> MTSSVLAALLSVSIMLVQLRAEANIGTGDNVLHRAALCGIIELAGKRAKLETALPNFQNELNSILELNMTAAEPTWLDQFRDKDDRSKPRDLTKQPLPKDTNWADHWTAWAKAALPLLNDETHQAKLKEYKLAGLQPEKLERARNTIRRLTAEAVAKAQDPTVAESTADLTTEEDLQKQINQAVYSKDTEPDDDFNGYTAFEGKASTNRQTICGSAVAGSKATNAMDALFCVCADDRTNGADAGKACVAGTAPGTGWNPGVTATPTGTMLQKVRKLCNTHGKTTLSAAAIEGRLTAVGNLLTRGSATSILGSFLATDCSGDQGSGMCVAYTEVTDAKGTPTKDIPWMQKLDSVRIKLQKHERAVEKLGKPQHDLKTILTLAKDPAYLQLASVGTRHLETTKQRVSNEQGK

Long-term immune evasion by the African trypanosome is achieved through repetitive cycles of surface protein replacement with antigenically distinct versions of the dense Variant Surface Glycoprotein (VSG) coat. The mature VSG proteins are attached to the cell surface by a GPI-anchor, and consist of two main regions: (1) a large, N-terminal domain (NTD) of roughly 300–400 amino acids that is most distal to the membrane and (2) a smaller, membrane-proximal C-terminal domain (CTD) spanning 80–120 amino acids beneath the NTD that harbors the GPI-anchor. Therefore, at the heart of antigenic variation in the African trypanosome are the NTDs of the VSGs. These large subdomains are elongated folds centered on a three-helix bundle scaffold.

VSG11 and VSG615 are related to VSG3 (the topologically-similar class of monomer/trimers with O-linked glycan PTMs), denoted as class B or N4 in the literature. NTD structures of VSG11 and VSG615 were solved to 1.23Å and 3.2Å resolution, respectively. Both reveal a fold similar to VSG3 as well as the presence of O-linked glycans on the top surface of the protein–one observed on VSG11 and two on VSG615. In addition, alignments of the VSG11WT-Iodine crystal form with the VSG11WT-Oil form show that the second helix of the three-helix bundle displays a significant conformational change in the region near the middle of the bundle, the helix becoming disordered and forming a random coil in one monomer while keeping helical structure in the other.> MSNISRQAYADMFGPTVGDKVRLADTELWIEVEDDLTTYGEEVKFGGGKVIRDGMGQGQMLAADCVDLVLTNALIVDHWGIVKADIGVKDGRIFAIGKAGNPDIQPNVTIPIGAATEVIAAEGKIVTAGGIDTHIHWICPQQAEEALVSGVTTMVGGGTGPAAGTHATTCTPGPWYISRMLQAADSLPVNIGLLGKGNVSQPDALREQVAAGVIGLKIAEDWGATPAAIDCALTVADEMDIQVAL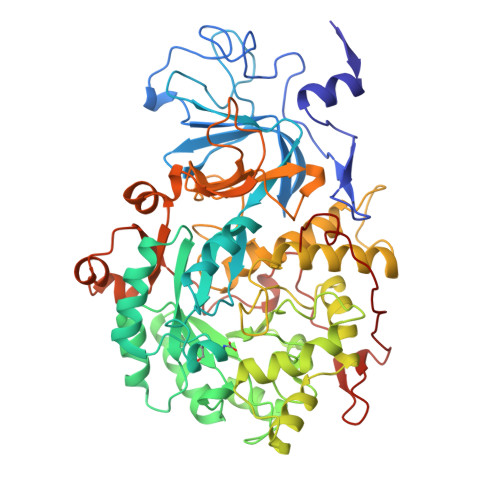HSDTLNESGFVEDTLAAIGGRTIHTFHTEGAGGGHAPDIITACAHPNILPSSTNPTLPYTLNTIDEHLDMLMVCHHLDPDIAEDVAFAESRIRRETIAAEDVLHDLGAFSLTSSDSQAMGRVGEVILRTWQVAHRMKVQRGALAEETGDNDNFRVKRYIAKYTINPALTHGIAHEVGSIEVGKLADLVVWSPAFFGVKPATVIKGGMIAIAPMGDINASIPTPQPVHYRPMFGALGSARHHCRLTFLSQAAAANGVAERLNLRSAIAVVKGCRTVQKADMVHNSLQPNITVDAQTYEVRVDGELITSEPADVLPMAQRYFLF>[4x]MHHHHHHGENLYFQGSEGEGVQLTAAQELMIQQLVAAQLQCNKR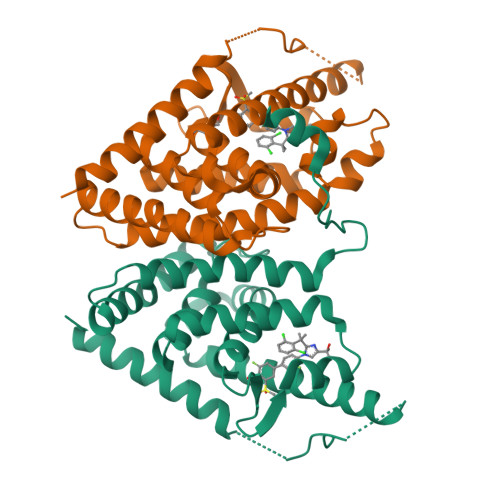SFSDQPKVTPWPLGADPQSRDARQQRFAHFTELAIISVQEIVDFAKQVPGFLQLGREDQIALLKASTIEIMLLETARRYNHETECITFLKDFTYSKDDFHRAGLQVEFINPIFEFSRAMRRLGLDDAEYALLIAINIFSADRPNVQEPGRVEALQQPYVEALLSYTRIKRPQDQLRFPRMLMKLVSLRTLSSVHSEQVFALRLQDKKLPPLLSEIWDVHE>HHHHHHMATRSPGVVISDDEPGYDLDLFAIPNHYAEDLERVFIPHGLIM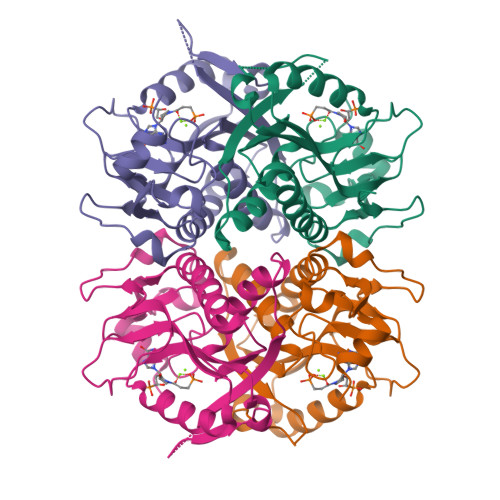DRTERLARDVMKEMGGHHIVALCVLKGGYKFFADLLDYIKALNRNSDRSIPMTVDFIRLKSYCNDQSTGDIKVIGGDDLSTLTGKNVLIVEDIIDTGKTMQTLLSLVRQYNPKMVKVASLLVKRTPRSVGYKPDFVGFEIPDKFVVGYALDYNEYFRDLNHVAVISETGKAKYKA[4x]GUANOSINE 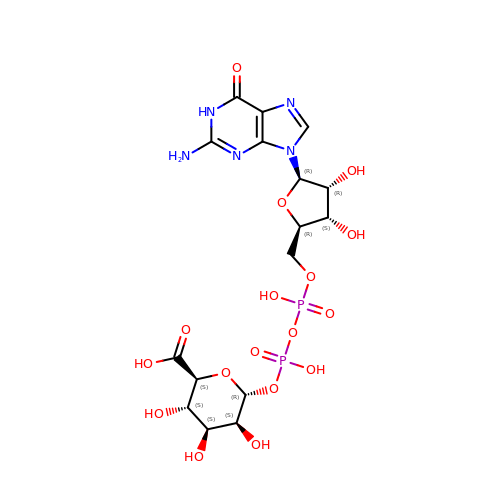5'-(TRIHYDROGEN DIPHOSPHATE), P'-D-MANNOPYRANOSYL ESTER | C16 H23 N5 O17 P2 | DNBSDUDYNPJVCN-ZXTXFPBHSA-N> MGPSLDFALSLLRRNIRQVQTDQGHFTMLGVRDRLAILPRHSQPGKTIWVEHKLINVLDAVELVDEQGVNLELTLVTLDTNEKFRDVTKFIPETITGASDATLIINTEHMPSMFVPVGDVVQYGFLNLSGKPTHRTMMYNFPTKAGQAGGVVTSVGKII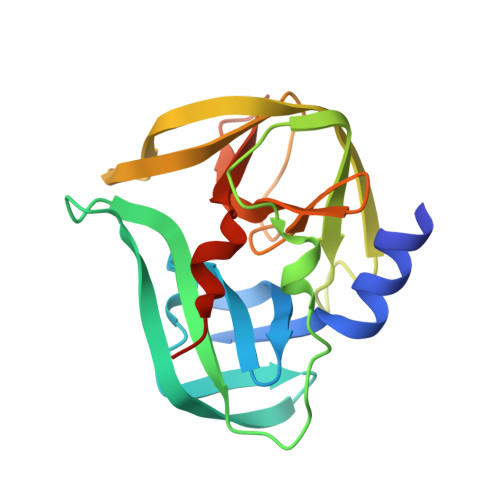GIHIGGNGRQGFCAGLKRGYFASEQHHHHHH> MKAQGETEDSERLSKMSSLLERLHAKFNQNRPWSETIKLVRQVMEKRVVMSSGGHQHLVSCLETLQKALKVTSLPAMTDRLESIARQNGLGSHLSASGTECYITSDMFYVEVQLDPAGQLCDVKVAHHGENPVSCPELVQQLREKNFEEFSKHLKGLVNLYNLPGDNKLKTKMYLALQSLEQDLSKMAIMYWKATNAAPLDKILHGSVGYLTPRSGGHLMNMKYYASPSDLLDDKTASPIILHEKNVPRSLGMNASVTIEGTSAMYKLPIAPLIMGSHPADNKWTPSFSAVTSANSVDLPACFFLKFPQPIPVSKAFVQKLQNCTGIPLFETPPTYLPLYELITQFELSKDPDPLPLNHNMRFYAALPGQQHCYFLNKDAPLPDGQSLQGTLVSKITFQHPGRVPLILNMIRHQVAYNTLIGSCVKRTILKEDSPGLLQFEVCPLSESRFSVSFQHPVNDSLVCVVMDVQDSTHVSCKLYKGLSDALICTDDFIAKVVQRCMSIPVTMRAIRRKAETIQADTPALSLIAETVEDMVKKNLPPASSPGYGMTTGNNPMSGTTTPTNTFPGGPITTLFNMSMSIKDRHESVGHGEDFSKVSQNPILTSLLQITGNGGSTIGSSPTPPHHTPPPVSSMAGNTKNHPMLMNLLKDNPAQDFSTLYGSSPLERQNSSSGSPRMEMCSGSNKAKKKKSSRVPPDKPKHQTEDDFQRELFSMDVDSQNPMFDVSMTADALDTPHITPAPSQCSTPPATYPQPVSHPQPSIQRMVRLSSSDSIGPDVTDILSDIAEEASKLPSTSDDCPPIGTPVRDSSSSGHSQSALFDSDVFQTNNNENPYTDPADLIADAAGSPNSDSPTNHFFPDGVDFNPDLLNSQSQSGFGEEYFDESSQSGDNDDFKGFASQALNTLGMPMLGGDNGEPKFKGSSQADTVDFSIISVAGKALGAADLMEHHSGSQSPLLTTGELGKEKTQKRVKEGNGTGASSGSGPGSDSKPGKRSRTPSNDGKSKDKPPKRKKADTEGKSPSHSSSNRPFTPPTSTGGSKSPGSSGRSQTPPGVATPPIPKITIQIPKGTVMVGKPSSHSQYTSSGSVSS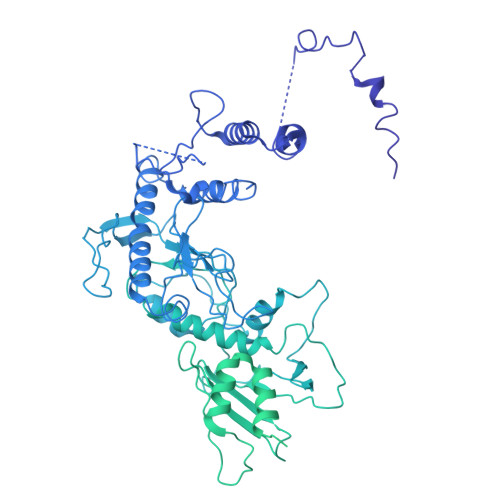SGSKSHHSHSSSSSSLASASTSGKVKSSKSEGSSSSKLSGSMYASQGSSGSSQSKNSSQTGGKPGSSPITKHGLSSGSSSTKMKPQGKPSSLMNPSISKPNISPSHSRPPGGSDKLASPMKPVPGTPPSSKAKSPISSGSSGSHVSGTSSSSGMKSSSGSASSGSVSQKTPPASNSCTPSSSSFSSSGSSMSSSQNQHGSSKGKSPSRNKKPSLTAVIDKLKHGVVTSGPGGEDPIDSQMGASTNSSNHPMSSKHNTSGGEFQSKREKSDKDKSKVSASGGSVDSSKKTSESKNVGSTGVAKIIISKHDGGSPSIKAKVTLQKPGESGGDGLRPQIASSKNYGSPLISGSTPKHERGSPSHSKSPAYTPQNVDSESESGSSIAERSYQNSPSSEDGIRPLPEYSTEKHKKHKKEKKKVRDKDRDKKKSHSMKPENWSKSPISSDPTASVTNNPILSADRPSRLSPDFMIGEEDDDLMDVALIGN>[2x]GGSMASMDFPQHSQHVLEQLNQQRQLGLLCDC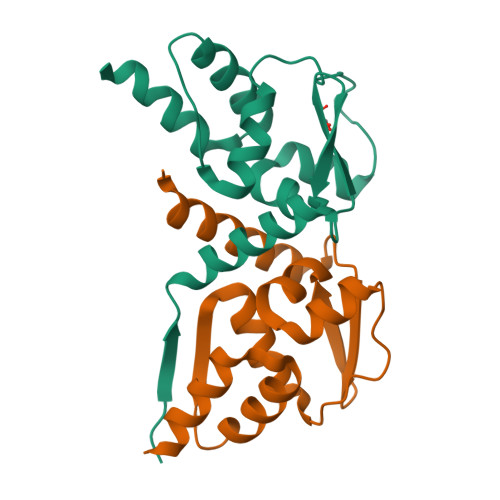TFVVDGVHFKAHKAVLAACSEYFKMLFVDQKDVVHLDISNAAGLGQVLEFMYTAKLSLSPENVDDVLAVATFLQMQDIITACHALKSLA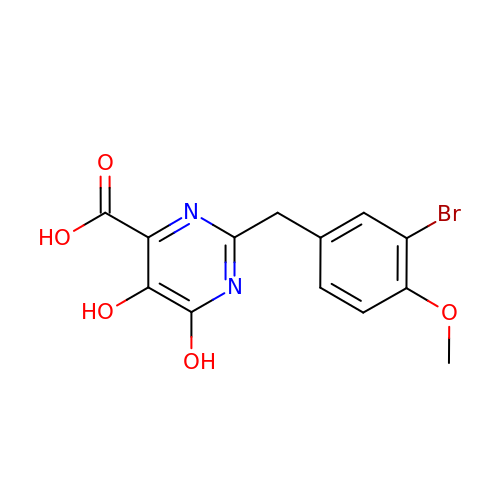2-(3-bromo-4-methoxybenzyl)-5,6-dihydroxypyrimidine-4-carboxylic acid | C13 H11 Br N2 O5 | LQQYBZYFFRDXNT-UHFFFAOYSA-N>[2x]GSHMKLCLVCSDEASGCHYGVL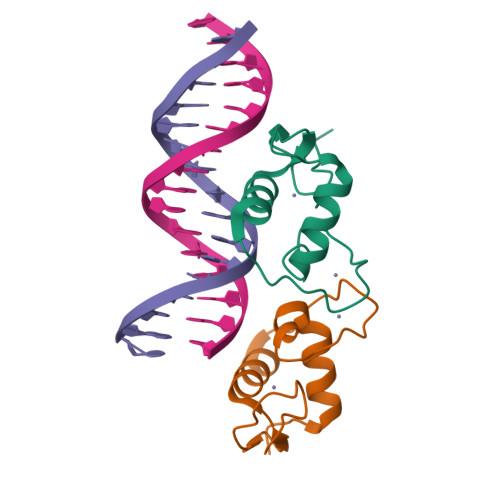TCGSCKVFFKRAVEGQHNYLCAGRNDCIIDKIRRKNCPACRYRKCLQAGMNLEARKTKKKIKGIQQATT>[2x]MNQEVRFSRLEPEQRKALLIEATLACLKRHGFQGASVRKICAEAGVSVGLINHHYDGKDALVAEAYLAVTGRVMRLLRGAIDTAPGGARPRLSAFFEASF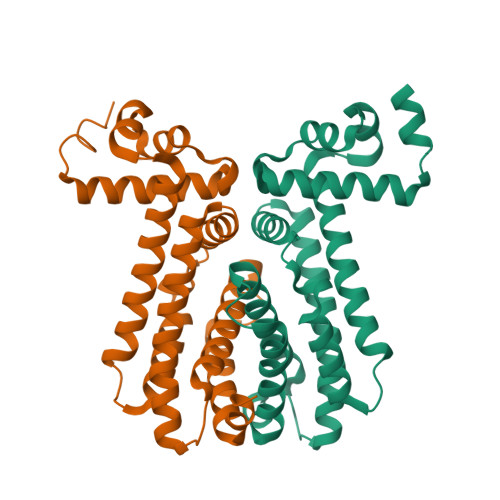SAELLDPQLLDAWLAFWGAVGSIEAIGRVHDHSYGEYRALLVGVLRQLAEEGGWADFDAELAAISLSALLDGLWLESGLNPATFTPRQGVQICEAWVDGLEAGAHRRFRRAMEAC> MTTLTLSEAAPLLKKEFREGRLIPFLGAGFSKPLKLPDGSQLIASLAKTLGFEPELFDMHGRFEQLAEFFAISAPNRLQRLVYEMSLSFDSAEAEA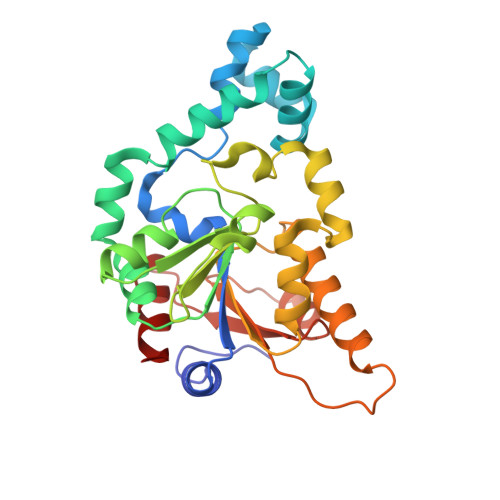LREKSPMHRALAALDWRTIYTTNYDKHVEGALRDAGKQAAVLASFADFQGPRARDVCEVIKFHGTLDQPDTIVLTESSYFQRMALDAPPDQRLRADLLANSFLFIGYSFSDTNIRYIWYRMNQLREQSQLGVKHSQARRCFFATHGAGLVQPDILQQWNIDVIQLDPTDKSASVARLLESIA4,4'[1,6-HEXANEDIYLBIS(OXY)]BISBENZENECARBOXIMIDAMIDE | C20 H26 N4 O2 | 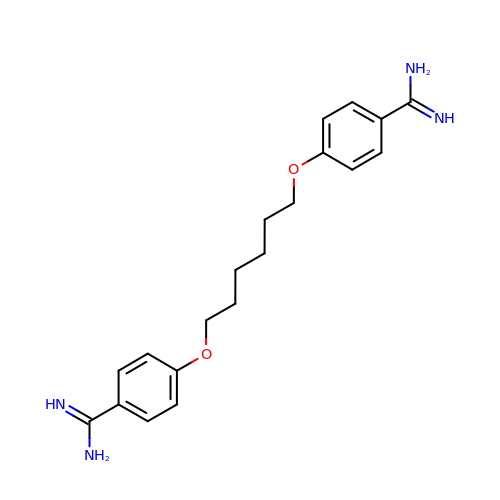OQLKNTOKMBVBKV-UHFFFAOYSA-N>MSKLASPQSVRALLERHGLFADKRFGQNFLVSEAHLRRIVEAARPFTGPVFEVGPGLGALTRALLEAGAEVTAIEKDLRLRPVLEETLSGLPVRLVFQDALLYPWEEVPQGSLLVANLPYHIATPLVTRLLKTGRFARLVFLVQKEVAERMTARPKTPAYGVLTLRVAHHAVAERLFDLPPGAFFPPPKVWSSLVRLTPTGALDDPGLFRLVEAAFGKRRKTLLNALAAAGYPKARVE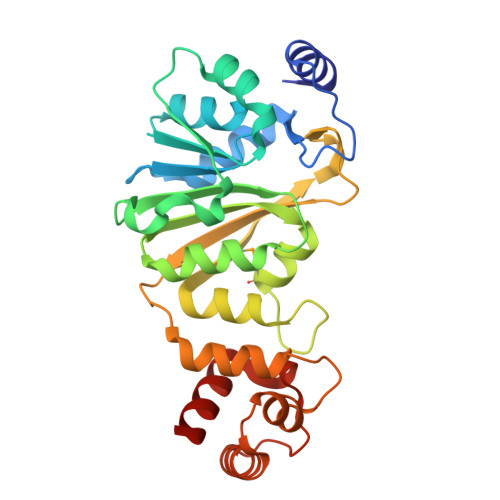EALRALGLPPRVRAEELDLEAFRRLREGLEGAV[2x]> MAKKTSSKGKLPPGPRPLPLLGNLLQMDRRGLLKSFLRFREKYGDVFTVHLGPRPVVMLCGVEAIREALVDKAEAFSGRGKIAMVDPFFRGYGVVFANGNRWKVLRRFSVTTMRDFGMGKRSVEERIQEEAQCLIEELRKSKG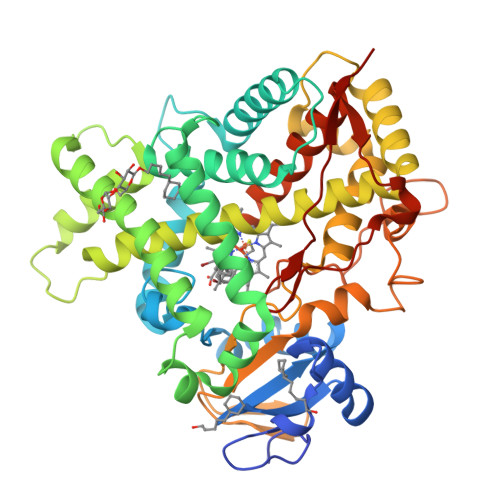ALMDPTFLFQSITANIICSIVFGKRFHYQDQEFLKMLNLFYQTFSLISSVFGQLFELFSGFLKHFPGAHRQVYKNLQEINAYIGHSVEKHRETLDPSAPRDLIDTYLLHMEKEKSNAHSEFSHQNLNLNTLSLFFAGTETTSTTLRYGFLLMLKYPHVAERVYREIEQVIGPHRPPELHDRAKMPYTEAVIYEIQRFSDLLPMGVPHIVTQHTSFRGYIIPKDTEVFLILSTALHDPHYFEKPDAFNPDHFLDANGALKKTEAFIPFSLGKRICLGEGIARAELFLFFTTILQNFSMASPVAPEDIDLTPQECGVGKIPPTYQIRFLPRHHHH> MKHHHHHHPMTTKQWGITPPISTAPATEQENALNTALINELKNQNLFESPAESEKRVKVLDELQQITTEFVKKVSLAKHMNEKMANEAGGKIFTYGSYRLGVYGPGSDIDTLVVVPKHVSRDNFFQDLEPMLREREEVTDLAAVPDAYVPIIKFKFLGISIDLIFARLSVPRVPRDLELSDNNLLKGVEERCVLSLNGTRVTDQILQLVPNRAVFKHALRAIKFWAQRRAIYANVVGFPGGVAWAMMV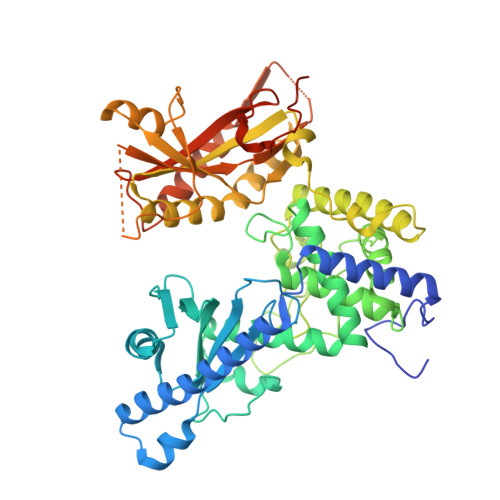ARICQLYPNAVSSVIVAKFFRILHQWNWPQPILLKPIEDGPLQVRIWNPKLYPSDKAHRMPIITPAYPSMCATHNITLSTQTIILREMVRAGEIADQIMVKALPWSALFQKHDFFHRYKHYLTITAAAKTAEAQLKWAGLVESKLRHLVTRLELVDAIALAHPFNKGFDKVYNCSSEEEAQQVASGVTLEVAYESTDHEKLANDTVNEEKADNTESKADGSENGEKQIFPVYTTTCYIGLELEKKKGHPIKRLDISWPTQEFYELCKKWDKYDDTLMNVFIKNTKNTALPDEVFEPGEERPKATKKRSTADTAHSTEQLKRQKVSTA> SRGELLLSLCYNPSANSIIVNIIKARNLKAMDIGGTSDPYVKVWLMYKDKRVEKKKTVTKKRNLNPIFNESFAFDIPTEKLRETTIIITVMDKDKLSRNDVIGKIYLSWKSGPGEVKHWKDMIARPRQPVAQWHQLKA

Members from the synaptotagmin family form a hierarchy of Ca2+ sensors and are believed to underlie at least in part the distinct Ca2+ dependencies of different forms of regulated secretion. Functional differentiation among synaptotagmins is expected to arise primarily from differences in the properties of the two C2 domains that form most of their cytoplasmic regions (referred to as C2A and C2B domains). In this context, the C2 domains of synaptotagmin-1 have been the subjects of particularly extensive study. Both domains form characteristic β-sandwich structures that bind three or two Ca2+ ions (C2A or C2B, respectively) through loops located at the top of the β-sandwich, and do not undergo substantial conformational changes upon Ca2+ binding. The relation between the functions of synaptotagmins-1 and-7 is particularly fascinating, as data obtained in chromaffin cells suggest that these two isoforms play at least partially redundant roles, and yet synaptotagmin-7 does not function as a Ca2+ sensor for synaptic vesicle exocytosis despite being enriched in synapses.

We describe the crystal structure of the Ca2+-bound synaptotagmin-7 C2B domain at 1.44 Å resolution, which is very similar to that of the synaptotagmin-1 C2B domain. Apart from this expected difference, the structure of the synaptotagmin-7 C2B domain is very similar to the crystal structure of the synaptotagmin-1 C2B domain. The r.m.s. deviation between 713 common atoms of the synaptotagmins-7 and -1 C2B domain is 0.71 Å, which is comparable to differences observed between structures of a given protein in different crystal forms. We observed three Ca2+ ions bound at the cup shape formed by the top loops of the synaptotagmin-7 C2B domain (loops 1–3). The three Ca2+ ions bound at the cavity formed by the top loops are coordinated by five aspartate and one serine side chains, as well as by three backbone carbonyl groups (the Ca2+-binding sites are numbered 1–3 as is common for C2 domains). In contrast, the C2B domain of synaptotagmin-1 was found to bind only two Ca2+ ions due to the absence of the serine side chain in loop 3 that helps to coordinate the third Ca2+ ion in the synaptotagmin-1 C2A domain (S235) and the synaptotagmin-7 C2B domain (S362). Note that this serine residue of loop 3 is not generally conserved in synaptotagmin C2B domains and hence binding of the third Ca2+ ion is an unusual feature of the synaptotagmin-7 C2B domain compared to other isoforms. We also observed a fourth Ca2+ ion bound outside of this region, but this site is not common in C2 domains and the Ca2+ ion is coordinated by only three protein ligands, suggesting that occupation of this site is due to the high Ca2+ concentration present in the crystallization conditions (20 mM) and is not physiologically relevant.> GSHMSNTQT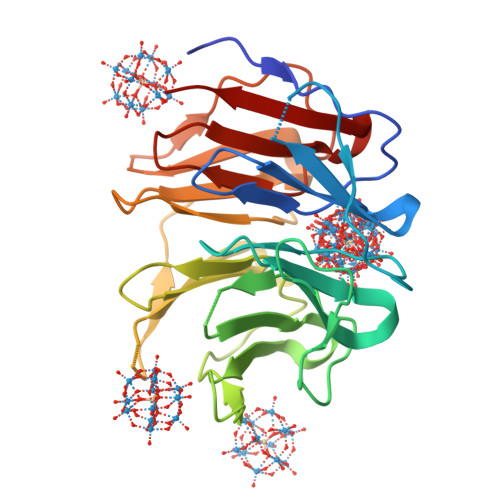VLPFTGLNRPSGVAVDSAGTVYVTDHGNNRVVKLAAGSNTQTVLPFTGLNTPSGVAVDSAGTVWVTDHGNNRVVKLAAGSNTQTVLPFTGLNRPSGVAVDSAGTVYVTDHGNNRVVKLAAGSNTQTVLPFTGLNTPSGVAVDSAGTVWVTDHGNNRVVKLAAGSNTQTVLPFTGLNRPSGVAVDSAGTVYVTDHGNNRVVKLAAGSNTQTVLPFTGLNTPSGVAVDSAGTVWVTDHGNNRVVKLAAG> ANAFLEELRPGSLERECKEEQCSFEEAREIFK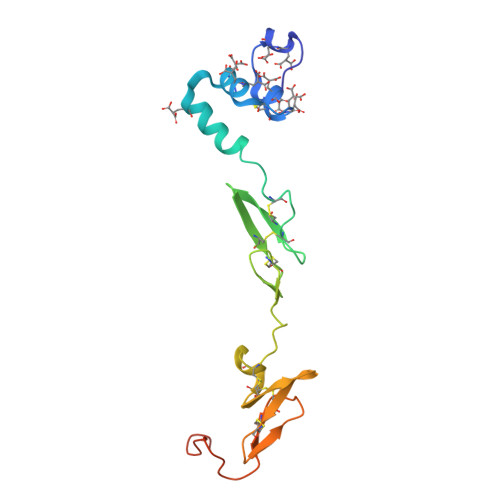DAERTKLFWISYSDGDQCASSPCQNGGSCKDQLQSYICFCLPAFEGRNCETHKDDQLICVNENGGCEQYCSDHTGTKRSCRCHEGYSLLADGVSCTPTVEYPCGKIPILEKRNASKPQGR> EKIAIRDFQVGDLVLIILDERHDNYVLFTVSPTLYFLHSESLPALDLKPGEGASGASRRPWVLGKVMEKEYCQAKKAQNRFKVPLGTKFYRVKAVSWNKKV

The formation of autophagosomes requires the hierarchical action of a number of conserved factors, including the upstream-acting ULK1 complex containing the scaffold protein FIP200 and the downstream-acting conjugation machinery, which catalyzes the conjugation of the ubiquitin-like ATG8 proteins to the head group of phosphatidylethanolamine on the isolation membrane. Crystal structure determination shows that the FIP200 CTR contains a dimeric globular domain that we designated the “Claw” for its shape. The interaction of p62 with FIP200 is mediated by a positively charged pocket in the Claw, enhanced by p62 phosphorylation, mutually exclusive with the binding of p62 to LC3B, and it promotes degradation of ubiquitinated cargo by autophagy. The Claw is constituted of a six stranded, mostly antiparallel β sheet and a short α-helix.

We also determined the crystal structure of the isolated Claw domain without the adjacent coiled-coil and obtained higher resolution diffraction from this material. Crystals of the isolated Claw diffracted to 1.56 Å, permitting a precise characterization of side-chain conformations and ions and waters of solvation. The isolated Claw crystallized with a monomer in the asymmetric unit; however, the unit cell contains a crystallographic 2-fold-related molecule that interacts through interface-1. Three sulfate ions from the crystallization medium were bound to the isolated Claw monomer at a location distal to the dimer interface-1 but overlapping with the putative FIR binding pocket. These sites are of interest as sulfates ions of crystallization often serve as markers of biologically relevant phosphate binding sites. Sulfate 1 is coordinated by the main chain amide and the side-chain hydroxyl of S1532 and the guanidino groups of R1573 and R1584. Sulfate 2 is also coordinated by the side chains of R1573 and R1584. Sulfate 3 is coordinated by both the main-chain NH and side chain of R1573 and is near the side chain of K1569. As compared to the structure of the CTR, which does not contain bound sulfate ions, R1573 moves by about 4 Å to engage the ions, while other residues in the pocket only move minimally. The proximity of these three sulfates was suggestive of a potential binding site for a tris-phosphorylated peptide segment, such as perhaps the tri-phosphorylated S365-S370 segment of p62.> FSIAVTGATGQLGGLVIQHLLKKVPASQIIAIVRNVEKA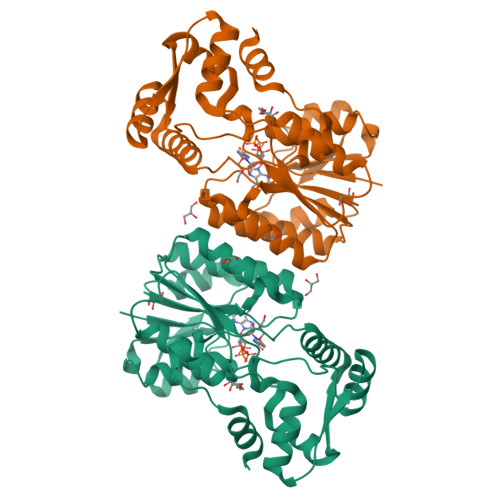STLADQGVEVRHGDYNQPESLQKAFAGVSKLLFISGPHYDNTLLIVQHANVVKAARDAGVKHIAYTGYAFAEESIIPLAHVHLATEYAIRTTNIPYTFLRNALYTDFFVNEGLRASTESGAIVTNAGSGIVNSVTRNELALAAATVLTEEGHENKTYNLVSNQPWTFDELAQILSEVSGKKVVHQPVSFEEEKNFLVNAGVPEPFTEITAAIYDAISKGEASKTSDDLQKLIGSLTPLKETVKQALKM>GPLGSSEQLKHCNGILKELLSKKHAAYAWPFYKPVDASALGLHDYHDIIKHPMDLSTV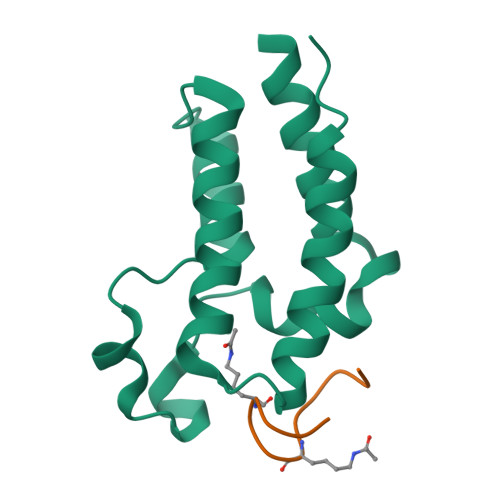KRKMENRDYRDAQEFAADVRLMFSNCYKYNPPDHDVVAMARKLQDVFEFRYAKMPD[2x];>[2x]WYGYWKVPKRKC>[2x]MEGVMGQVEKRPISTIVFIVAMQKEAQPLINRLRLVEEVNTPFPKEVTWIMFKGMYKDLNINIVCPGKDSTLGVESVGTVPASLVTYASILAIQPDLIINAGTAGGFKAKGACISDVYVVSTVAFHDRRIPVPVLDIYGV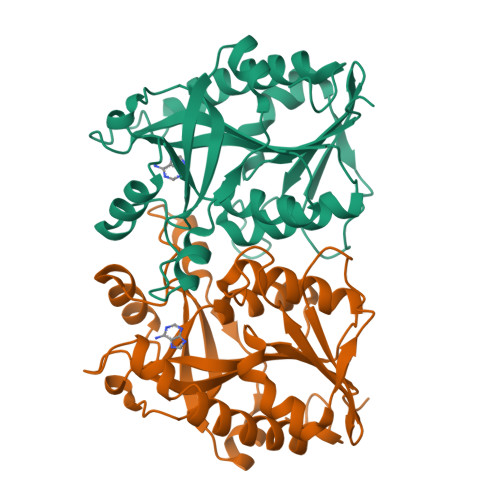GMRNTFPTPNLIKELNLKVGRLSTGDSMDMSPHDEESITANDATVKDMEGAAVAYVADIFKVPTILIKGVTDIVDGNRPTSEEFLENLAAVTAKLDESLTKVIDFISGKCLSDL[2-(hexylamino)ethane-1,1-diyl]bis(phosphonic acid) | C8 H21 N O6 P2 | 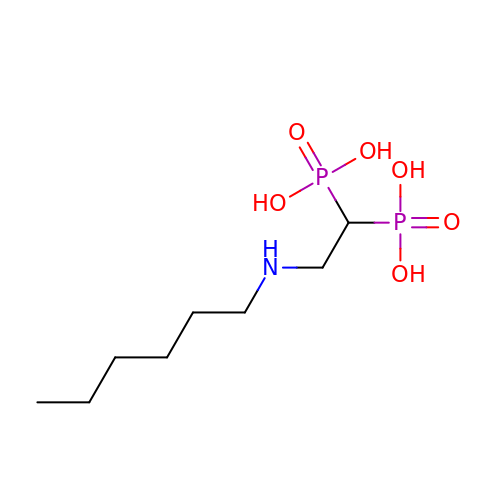QDLXIUDMSHZYCG-UHFFFAOYSA-N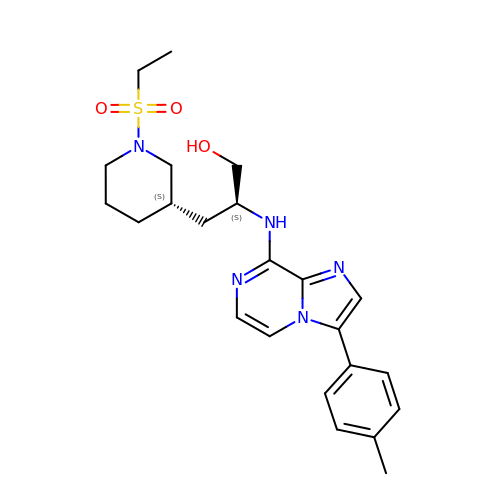(2S)-3-[(3S)-1-(ethylsulfonyl)piperidin-3-yl]-2-{[3-(4-methylphenyl)imidazo[1,2-a]pyrazin-8-yl]amino}propan-1-ol | C23 H31 N5 O3 S | LSSLQEALPIQUKR-ICSRJNTNSA-N> TAYYAQALQSVPETQVSQLDNGVRVASEQSSQPTCTVGVWIDAGSRYESEKNNGAGYFLEHLAFKGTKNRPQNALEKEVESMGAHLNAYSSREHTAYYIKALSKDVPKAVELLADIVQNCSLEDSQIEKERDVIVRELQENDTSMREVVFNYLHATAFQGTGLAQSVEGPSENIRKLSRADLTEYLSTHYTAPRMVLAAAGGVEHQQLLELAQKHFGGVPFTYDDDAVPTLSKCRFTGSQIRHREDGLPLAHVAIAVEGPGWAHPDLVALQVANAIIGHYDRTYGGGLHSSSPLASIAVTNKLCQSFQTFSICYSETGLFGFYFVCDRMSIDDMMFVLQGQWMRLCTSISESEVLRGKNFLRNALVSHLDGTTPVCEDIGRELLTYGRRIPLEEWEERLAEVDARMVREVCSKYIYDQCPAVAGPGPIEQLPDYNRIRSGMFWLRF;> PPHPQDLEITKLPNGLVIASLENYSPGSTIGVFIKAGSRYENSSNLGTSHLLRLASSLTTKGASSFKITRGIEAVGGKLSVESTRENMAYTVECLRDDVEILMEFLLNVTTAPEFRPWEVADLQPQLKIDKAVAFQNPQTHVIENLHAAAYRNALADSLYCPDYRIGKVTSVELHDFVQNHFTSARMALVGLGVSHPVLKNVAEQLLNIRGGLGLSGAKAKYRGGEIREQNGDSLVHAAIVAESAAIGGAEANAFSVLQHVLGANPHVKRGLNATSSLYQAVAKGVHNPFDVSAFNASYSDSGLFGFYTISQAAYAGQVIKAAYNQVKTIAQGNVSNENVQAAKNKLKAKYLMSVESSEGFLEEVGSQALAAGSYNPPSTVLQQIDAVADADVIKAAKKFVSRQKSMAASGNLGHTPFVDEL;> MAPNIRKSHPLLKMINNSLIDLPAPSNISAWWNFGSLLAVCLMTQILTGLLLAMHYTADTSLAFSSVAHTCRNVQYGWLIRNLHANGASFFFICIFLHIGRGLYYGSYLYKETWNTGVILLLTLMATAFVGYVLPWGQMSFWGATVITNLFSAIPYIGHTLVEWAWGGFSVDNPTLTRFFALHFLLPFAIAGITIIHLTFLHESGSNNPLGISSDSDKIPFHPYYSFKDILGLTLMLTPFLTLALFSPNLLGDPENFTPANPLVTPPHIKPEWYFLFAYAILRSIPNKLGGVLALAASVLILFLIPFLHKSKQRTMTFRPLSQTLFWLLVANLLILTWIGSQPVEHPFIIIGQMASLSYFTILLILFPTIGTLENKMLNY;> SDLELHPPSYPWSHRGPLSSLDHTSIRRGFQVYKQVCSSCHSMDYVAYRHLVGVCYTEDEAKALAEEVEVQDGPNEDGEMFMRPGKLSDYFPKPYPNPEAARAANNGALPPDLSYIVRARHGGEDYVFSLLTGYCEPPTGVSVREGLYFNPYFPGQAIGMAPPIYNDVLEFDDGTPATMSQVAKDVCTFLRWAAEPEHDHRKRMGLKMLLMMGLLVPLVYYMKRHKWSVLKSRKLAYRPPK;> SHTDIKVPNFSDYRRPPDDYSTKSSRESDPSRKGFSYLVTAVTTLGVAYAAKNVVTQFVSSMSASADVLAMSKIEIKLSDIPEGKNMAFKWRGKPLFVRHRTKKEIDQEAAVEVSQLRDPQHDLERVKKPEWVILIGVCTHLGCVPIAN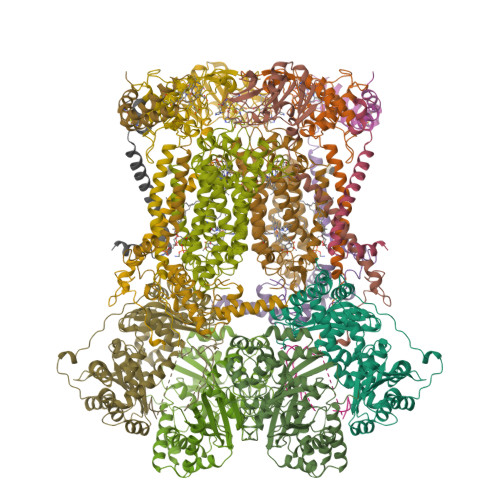AGDFGGYYCPCHGSHYDASGRIRKGPAPLNLEVPSYEFTSDDMVIVG;> AGRPAVSASSRWLEGIRKWYYNAAGFNKYGLMRDDTIYENDDVKEAIRRLPENLYDDRMFRIKRALDLNMRQQILPKEQWTKYEEDVPYLEPYLKEVIRERKEREEWDK;> GRQFGHLTRVRHLITYSLSPFEQRPFPHYFSKGVPNVWRRLRACILRVAPPFLAFYLLYTWGTQEFEKSKRKNPAAYVNDR;> GDPKEEEEEEEELVDPLTTVREQCEQLEKCVKARERLELCDERVSSRSQTEEDCTEELFDFLHARDHCVAHKLFNSLK;> VAPTLTARLYSLLFRRTSTFALTIVVGALLFERAFDQGADAIYEHINEGKLWKHIKHKYENK> MSQVTDMRSNSQGLSLTDSVYERLLSERIIFLGSEVNDEIANRLCAQILLLAAEDASKDISLYINSPGGSISAGMAIYDTMVLAPCDIATYAMGMAASMGEFLLAAGTKGKRYALPHARILMHQPLGGVTGSAADIAIQAEQFAVIKKEMFRLNAEFTGQPIERIEADSDRDRWFTA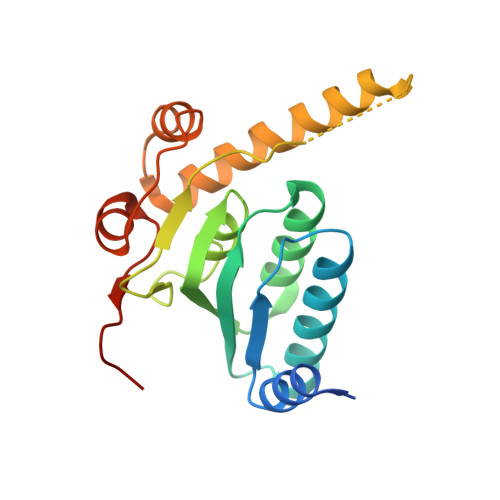AEALEYGFVDHIITRAHVNGEAQ>[4x]GAMAGKKVLIVYAHQEPKSFNGSLKNVAVDELSRQGCTVTVSDLYAMNFEPRATDKDITGTLSNPEVFNYGVETH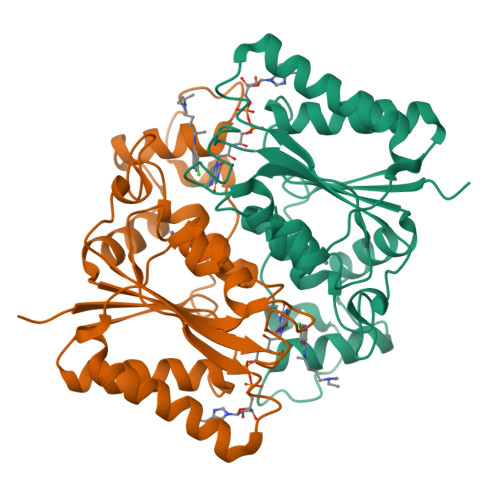EAYKQRSLASDITDEQKKVREADLVIFQFPLYWFSVPAILKGWMDRVLCQGFAFDIPGFYDSGLLQGKLALLSVTTGGTAEMYTKTGVNGDSRYFLWPLQHGTLHFCGFKVLAPQISFAPEIASEEERKGMVAAWSQRLQTIWKEEPIPCTAHWHFGQ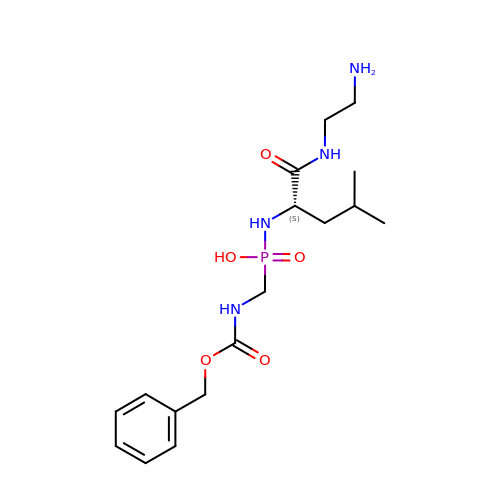~{N}-[(2~{S})-1-(2-azanylethylamino)-4-methyl-1-oxidanylidene-pentan-2-yl]-(phenylmethoxycarbonylaminomethyl)phosphonamidic acid | C17 H29 N4 O5 P | PVGHXKGUTYHASF-HNNXBMFYSA-N>[2x]SHMNKDNLRSPICCILGHVDTGKTKLLDKIRQTN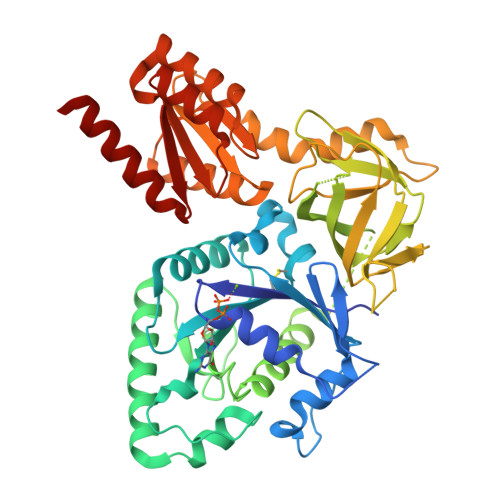VQEGEAGGITQQIGATYFPVEAIKQKTAVVNKDGKFEFKVPGLLIIDTPGHESFSNLRSRGSSLCNIAILVVDIMHGLEPQTIESLRLLRERKTPFVVALNKIDRLYGWKKIENNGFRESFALQNKAVQNEFRNRLDQVKLQFAEQGFNSELFYENKNFARYVSLVPTSAHTGEGIPDMLKLIVQLCQERMASSLMYLSELQATVLEVKAIEGFGVTIDVILSNGILREGDRIVLCGLEGPIKTNIRALLTPAPMRELRIKGQYIHHKEVKAAQGVKISAPGLEGAIAGSRLLVVGPDDDEEELEEEVESDLQSLFSRVEKTGKGVSVQASTLGSLEALLDFLKDCKIPVANVGIGPVYKRDVMQCGIMLEKAPDYAVMLCFDVKVDKEAQQYADENGIKIFTADIIYHLFDQFTKHMQEQLE> MGCVRVRTGCRIRCVRASFTYTQAQMYARYRTRSRFYKRPEKMLKAYNVSPNLLRLPKVKPGLLKGIYTDEKIDLRDRERLELVESIRHPKERDFYQDHTYHNQWIARDLESHQKIQIAGRYPYFSPDYEIKPWIWYPGDTVEVVSGEGAGQRGAIIAVVKYKNEILVQNVNVQDVVIPASETRPEQVVQREHPISVLRVRHVDPSTNQLCHLEIVKVRNKETGELEERRISLESGALLPIPAPEETVEAGDPLKDTAIQDADEETYDREKEMPLLVVRRLQAME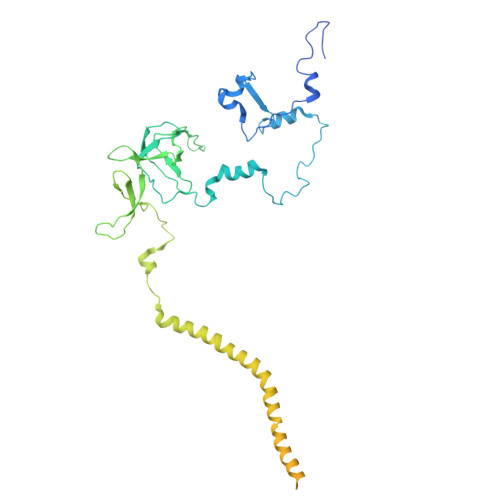NYFVDSLQKSHEYHKALQMRNAQDMQTFQKDVLVRATEKLAAAAAVAGHGAMAEAGSQAASVATESSQAGDAEEDAVKGTITVETVVAEVLKSEQRFRSDAAAPGVPGWWQNMIDAYVSVLEEEEATIEAEAAAQAQAAEADRRAEQLMADATAEAGQSMEEDGTMEGGDEDLDEQDGDLDEDASRSDRSK> MAHHHHHHDYGIPTTENLYFQGSNPNYCFAGKTSSISDLKEVPRKNITLIRGLGHGAFGEVYEGQVSGMPNDPSPLQVAVKTLPEVYSEQDELDFLMEALIISKFNHQNIVRCIGVSLQSLPRFI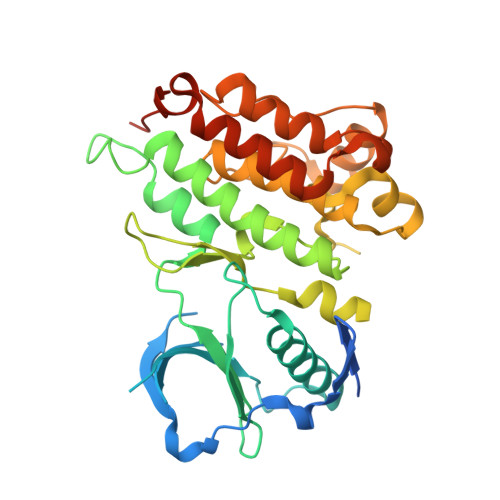LLELMAGGDLKSFLRETRPRPSQPSSLAMLDLLHVARDIACGCQYLEENHFIHRDIAARNCLLTCPGPGRVAKIGDFGMARDIYRASYYRKGGCAMLPVKWMPPEAFMEGIFTSKTDTWSFGVLLWEIFSLGYMPYPSKSNQEVLEFVTSGGRMDPPKNCPGPVYRIMTQCWQHQPEDRPNFAIILERIEYCTQDPDVINTALPIEYGPLVEEEEKV>GAMDMKTLTTISGHSKDNLALLKCLQGETKEKEFEISNVLPNHKMKEKLFRENKLKIDIDIEKDIFNYSRKNIQKIEFMPVNRLISQSEIDGIIGTLKEVL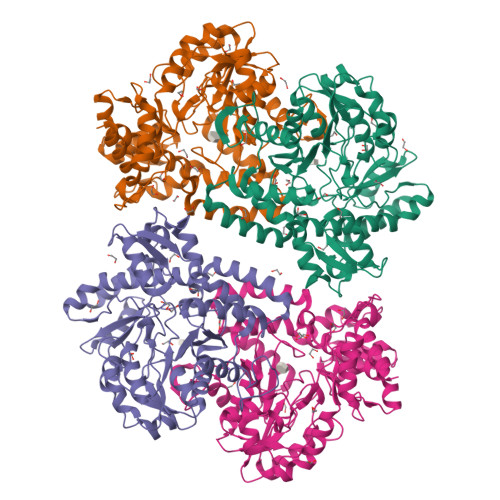PTGQFTSGPFSKKLEEVIGDYLNKKYVIATSSGTDALMVSLLSIGIQPGDEVIMPANSFAATENAVLAIGAKPVFVDIDHKSYCIDPLKIEEAITQKTKCILPVHLYGKQCDMKRIREIADVYQLRIIEDACQAIGSSNLGEYGDIIILSFNPYKNFGVCGKAGAIVTNNENLAIRCNQYSYHGFEVDKKNKKVLDFGFNSKIDNLQAAIGLERIKFLSYNNLKRVFLAQRYIRNLKELEDRELIKLPRMTEDNVWHLFPIRIINGRRDEVKNKLYQLYNIETDIYYPVLSHKHNTKLVKKNYMQDTLLNTEQVHKEILHLPLHPNMLLEEQNFVLEGLINVNK[4x]> QDPCSNCPAGTFCDNNRNQICSPCPPNSFSSAGGQRTCDICRQCKGVFRTRKECSSTSNAECDCTPGFHCLGAGCSMCEQDCKQGQELTKKGCKDCCFGTFNDQKRGICRPWTNCSLDGKSV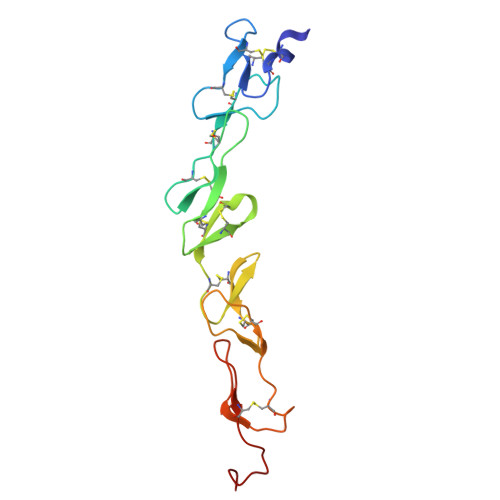LVNGTKERDVVCGPSPENLYFQ> MPKLVTWMNNQRVGELTKLANGAHTFKYAPEWLASRYARPLSLSLPLQRGNITSDAVFNFFDNLLPDSPIVRDRIVKRYHAKSRQPFDLLSEIGRDSVGAVTLIPEDETVTHPIMAWEKLTEARLEEVLTAYKADIPLGMIREENDFRISVAGAQEKTALLRIGNDWCIPKGITPTTHIIKLPIGEIRQPNATLDLSQSVDNEYYCLLLAKELGLNVPDAEIIKAGNVRALAVERFD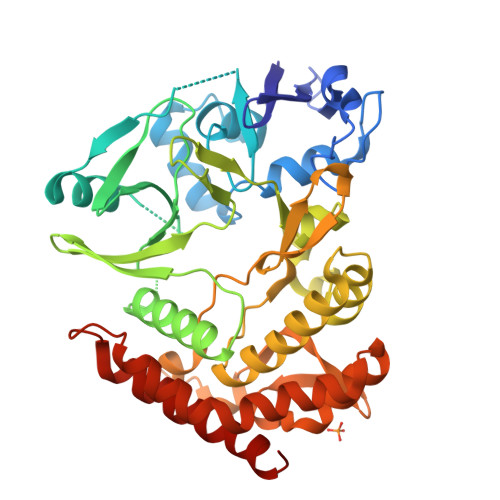RRWNARRTVLLRLPQEDMCQTFGLPSSVKYESDGGPGIARIMAFLMGSSEALKDRYDFMKFQVFQWLIGATDGHAKNFSVFIQAGGSYRLTPFYDIISAFPVLGGTGIHISDLKLAMGLNASKGKKTAIDKIYPRHFLATAKVLRFPEVQMHEILSDFARMIPAALDNVKTSLPTDFPENVVTAVESNVLRLHGRLSREYGSK>MASLLKVDQEVKLKVDSFRERITSEAEDLVANFFPKKLLELDSFLKEPILNIHDLTQIHSDMNLPVPDPILLTNSHDGLDGPTYKKRRLDECEEA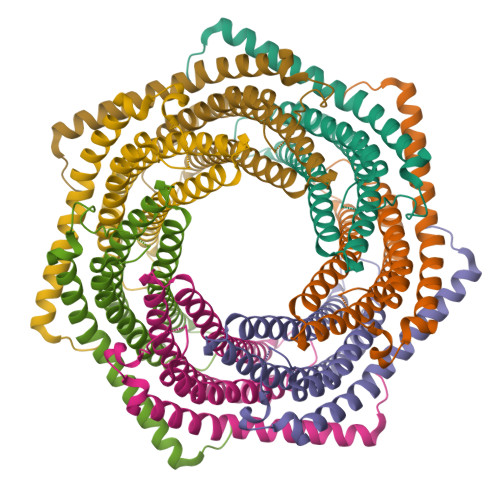FQGTKVFVMPNGMLKSNQQLVDIIEKVKPEIRLLIEKCNTVKMWVQLLIPRIEDGNNFGVSIQEETVAELRTVESEAASYLDQISRYYITRAKLASKIAKYPHVEDYARTVTEIDEKEYISLRLIISELRNQYVTLHDMILKNIEKIKRPRSSNAETLY[7x]> MSEGVEAIVANDNGTDQVNGNRTGKDNEEHDGSTGSNLSNFLWHGGSVWDAWFSCASNQVAQVLLTLPYSFSQLGMLSGIVLQIFYGLLGSWTAYLISVLYVEYRARKEKEGKSFKNHVIQWFEVLDGLLGSYWKALGLAFNCTFLLFGSVIQLIACASNIYYINDHLDKRTWTYIFGACCATTVFIPSFHNYRIWSFLGLGMTTYTAWYLAIASIIHGQAEGVKHSGPTKLVLYFTGATNILYTFGGHAVTVEIMHAMWKPQKFKYIYLMATLYVFTLTIPSAAAVYWAFGDALLDHSNAFSLMPKNAWRDAAVILMLIHQFITFGFACTPLYFVWE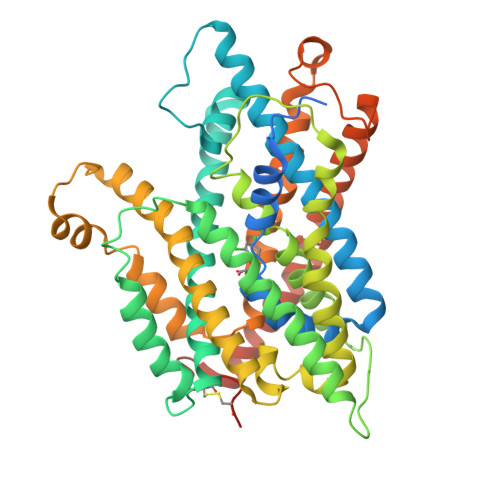KVIGMHDTKSICLRALARLPVVIPIWFLAIIFPFFGPINSAVGALLVSFTVYIIPSLAHMLTYRSASARQNAAEKPPFFMPSWTAMYVLNAFVVVWVLIVGFGFGGWASVTNFVRQVDTFGLFAKCYQCKPAAAAAHAPVSALHHRL>[2x]GSGSSSPLPKVAHNLGFYFSPDLTQFAKLPVELAPHWPVVTTQNNEKWPDRLVASLRPIHKYSRACIGAGYMVGPSVFLGTPGVVSYYLTKFVKGEAQLLPETVFST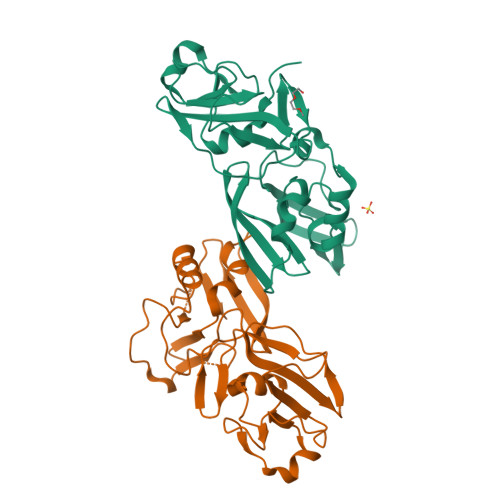GRIEVDCREYLDDREREVAASLPHAFIGDVKGTTVGGCHHVTSRYLPRVLPKESVAVVGVSSPGKAAAALCTLTDVYLPDLEAYLHPETQSKCWKMMLDFKEVRLMVWRDKTAYFQLE> GGGGGGMNVFNTASDEDIKKGLASDVYFERTISAIGDKCNDLRVAMEATVSGPLDTWINFTGLDEVLKLLEGLDVDLYAIPEGTILFPRDANGLPVPFIRVEGRYCDFGMYETAILGFICQASGISTKASKVRLAAGDSPF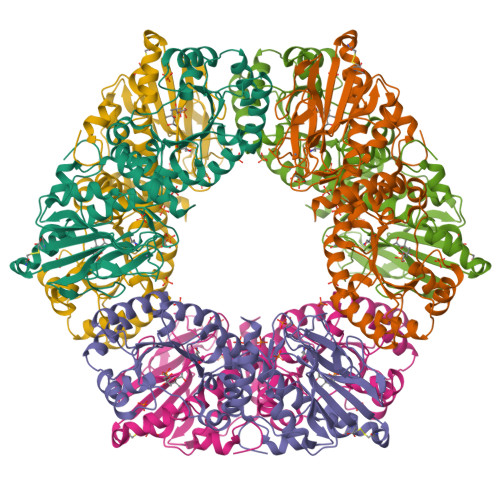FSFGIRRMHPAISPMIDRSAYIGGADGVSGILGAKLIDQDPVGTMPHALSIMLGDEEAWKLTLENTKNGQKSVLLIDTYMDEKFAAIKIAEMFDKVDYIRLDTPSSRRGNFEALIREVRWELALRGRSDIKIMVSGGLDENTVKKLREAGAEAFGVGTSISSAKPFDFAMDIVEVNGKPETKRGKMSGRKNVLRCTSCHRIEVVPANVQEKTCICGGSMQNLLVKYLSHGKRTSEYPRPKEIRSRSMKELEYFKDIS> MENGVCKSYKSVALVVGVTGIVGSSLAEVLKLPDTPGGPWKVYGVARRPCPVWLAKKPVEYIQCDVSDNQETISKLSPLKDITHIFYVSWIGSEDCQTNATMFKNILNSVIPNASNLQHVCLQTGIKHYFGIFEEGSKVVPHDSPFTEDL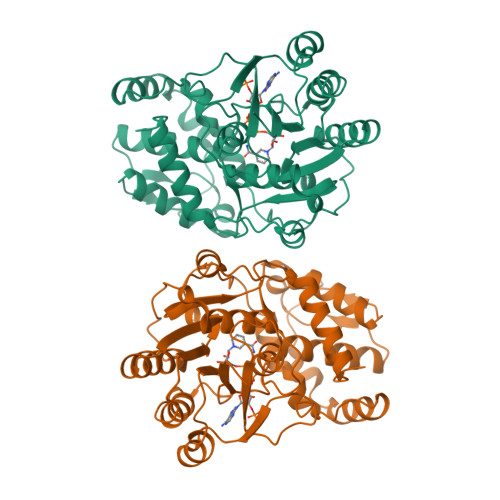PRLNVQNFYHDLEDILYEETGKNNLTWSIHRPALVFGFSPCSMMNIVSTLCVYATICKHENKALVYPGSKNSWNCYADAVDADLVAEHEIWAAVDPKAKNQVLNCNNGDVFKWKHIWKKLAEEFGIEMVGYVEGKEQVSLAELMKDKDQVWDEIVKKNNLVPTKLKEIAAFWFADIAFCSENLISSMNKSKELGFLGFRNSMKSFVSCIDKMRDYRFIP> MENSARQVAQDTRELHLLQHIKSDQSYIYVFVFLYYRDHSVRVWKLTNPVSISETLDYDDLINNVNRCKSAREPAIYYREGITGNDAGDSIIDKAYCEPVSFMIVACGDVDIQTIEVNIQGYDEIEGVGILDSNVTPPYAITATKFERK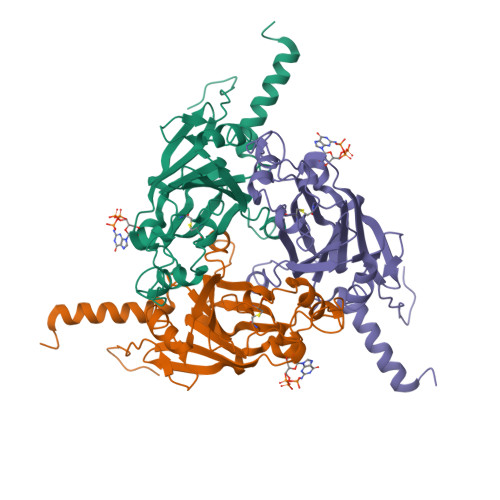TSGGYIFYTYCGLFGHGDRGHPTMAVGVEKKNRNAFGRMHPMYVAANYKRRNFWAKKDWWFPTEGQMVEQFIKQQSIPYVTADNVMIAPCVREIRHHAHY[(2~{R})-1-[[(1~{R},5~{S})-6,6-dimethyl-2-bicyclo[3.1.1]hept-2-enyl]methyl]pyrrolidin-2-yl]methanol 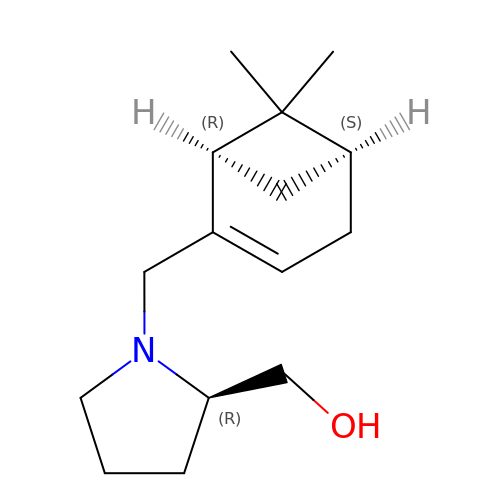| C15 H25 N O | MTWNYZLGPQWNAM-MJBXVCDLSA-N>GGGILPAPEKSSKVSEQLKCCSGILKEMFAKKHAAYAWPFYKPVDVEALGLHDYCDIIKHPMDMSTIKSKLEAREYRDAQEFGADVRLMFSNCYKYNPPDHE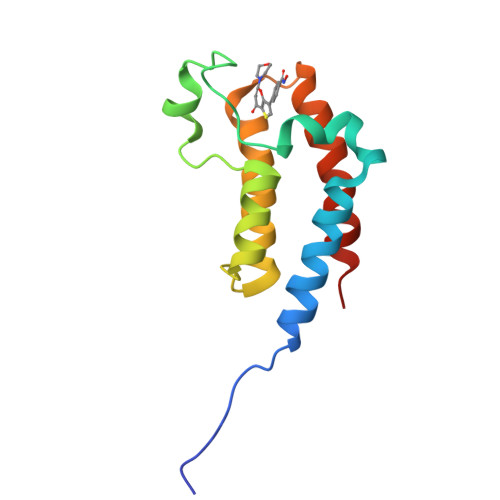VVAMARKLQDVFEMRFAKMPDE[2x]(4R,4a'R,10a'S)-8'-(2-fluoropyridin-3-yl)-4a'-methyl-3',4',4a',10a'-tetrahydro-2'H-spiro[1,3-oxazole-4,10'-pyrano[3,2-b]chromen]-2-amine 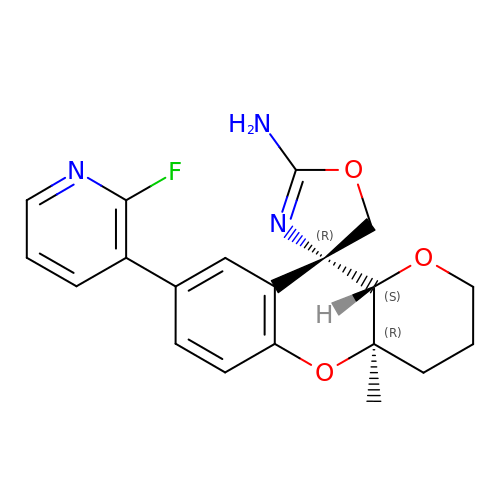| C20 H20 F N3 O3 | DMNHLGOPJBTFQJ-RLLQIKCJSA-N>[7x]MALIGQTLPSLLDIYNRTDKNGRIARIVEQLAKTNDILTDAIYVPCNDGSKHKTTIRAGIPEPVWRRYNQGVQPTKTQTVPVTDTTGMLYDLGFVDKALADRSNNAAAFRVSENMGKLQGFNNKVARYSIYGNTDAEPEAFMGLAPRFNTLSTSKAASAENVFSAGGSGSTNTSIWFMS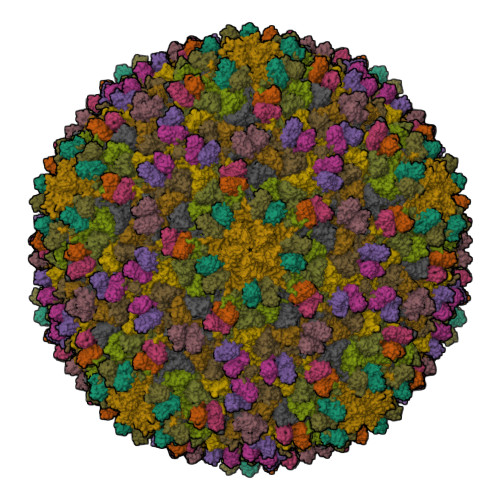WGENTAHMIYPEGMVAGFQHEDLGDDLVSDGNGGQFRAYRDEFKWDIGLSVRDWRSISRICNIDVTTLTKDASTGADLISMMVDAYYARDVAMLGDGKEVIYANKTIHAWLHKQAMNAKNVNLTIEEYGGKKIVSFLGIPIRRVDAILNTESAVTA;>MKTVNMKTGTDSFVGEDGKPETKDQYPWGLRITLDNESLQRLGLNAKSLPAVGDSVSVMAMANVCSVSTRTTDHGEDNYVELQITDIGLAPQKRDDAKELKDAFYPDGEDD[7x]>[2x]GPSQPKVPEWVNTPSTCCLKYYEKVLPRR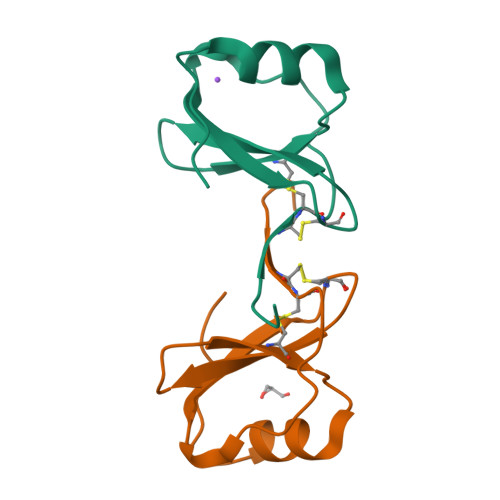LVVGYRKALNCHLPAIIFVTKRNREVCTNPNDDWVQEYIKDPNLPLLPTRNLSTVKIITAKNGQPQLLNSQ>[2x]MSREEVESLIQEVLEVYPEKARKDRNKHLAVNDPAVTQSKKCIISNKKSQPGLMTIRGCAYAGSKGVVWGPIKDMIHISHGPVGCGQYSRAGRRNYYIGTTGVNAFVTMNFTSDFQEKDIVFGGDKKLAKLIDEVETLFPLNKGISVQSECPIGLIGDDIESVSKVKGAELSKTIVPVRCEGFRGVSQSLGHHIANDAVRDWVLGKRDEDTTFASTPYDVAIIGDYNIGGDAWSSRILLEEMGLRCVAQWSGDGSISEIELTPKVKLNLVHCYRSMNYISRHMEEKYGIPWMEYNFFGPTKTIESLRAIAAKFDESIQKKCEEVIAKYKPEWEAVVAKYRPRLEGKRVMLYIGGLRPRHVIGAYEDLGMEVVGTGYEFAHNDDYDRTMKEMGDSTLLYDDVTGYEFEEFVKRIKPDLIGSGIK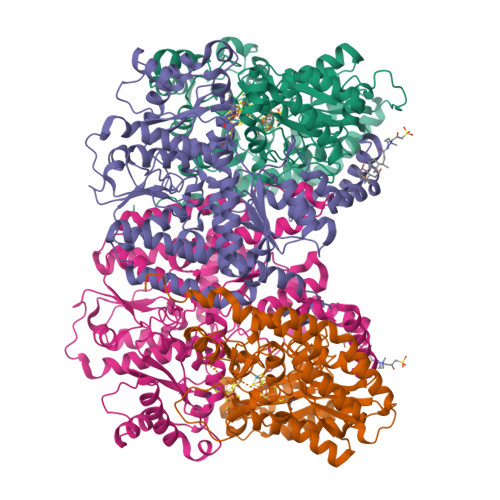EKFIFQKMGIPFREMHSWDYSGPYHGFDGFAIFARDMDMTLNNPCWKKLQAPWE;>[2x]SQQVDKIKASYPLFLDQDYKDMLAKKRDGFEEKYPQDKIDEVFQWTTTKEYQELNFQREALTVNPAKACQPLGAVLCALGFEKTMPYVHGSQGCVAYFRSYFNRHFREPVSCVSDSMTEDAAVFGGQQNMKDGLQNCKATYKPDMIAVSTTCMAEVIGDDLNAFINNSKKEGFIPDEFPVPFAHTPSFVGSHVTGWDNMFEGIARYFTLKSMDDKVVGSNKKINIVPGFETYLGNFRVIKRMLSEMGVGYSLLSDPEEVLDTPADGQFRMYAGGTTQEEMKDAPNALNTVLLQPWHLEKTKKFVEGTWKHEVPKLNIPMGLDWTDEFLMKVSEISGQPIPASLTKERGRLVDMMTDSHTWLHGKRFALWGDPDFVMGLVKFLLELGCEPVHILCHNGNKRWKKAVDAILAASPYGKNATVYIGKDLWHLRSLVFTDKPDFMIGNSYGKFIQRDTLHKGKEFEVPLIRIGFPIFDRHHLHRSTTLGYEGAMQILTTLVNSILERLDEETRGMQATDYNHDLVR>MRCLAAGVHYKTLIVICALLSLLTVLLWNKCTSEKALRFLPQHPQPPPSPKIDSHPQQPQPPEPPPVVGGVRYEEIDCLINDDATIKGRREGSEVYMPFSWMEKYFEVYGKVVQYDGYDRFEFSHSYSKVYAQREQYHPNGVFMSFEGYNVEVRDRVKCISGVEGVPLSTQWGPQGYFYAIQIAQYGLSHYSKNLTERPPHVEVYDTAEERDSRSSAWTVPKGCSLTRVYDKTRATSVREFSAPENSEGVSLPLGNTKDFIISFDLKFTSNGSVSVILETTEKGPPFVIHYVTTTQLILLKDRDITYGIGPRTTWTTVTRDLLTDLRKGIGLSNTKAVKAT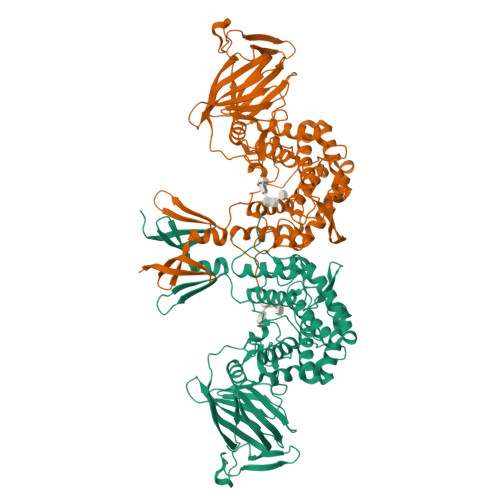KTMPRRVVKLVVHGTGTIDNITISTTSHMAAFYAASDWLVRNQDERGGWPIMVTRKLGEGFRALEPGWYSAMAQGQAMSTLVRAYLMTKDDRYLKAALRATGPFKLPSEQHGVKAVFMNKYDWYEEYPTIPSSFVLNGFIYSLIGLFDLAQTAGEKLGRDAGQLYSKGMESLKVMLPLYDTGSGTIYDLRHFILGTAPNLARWDYHTTHINQLQLLGTIDNSPIFRDSVKRWKSYLKGGRAKHN[2x]>NEFSASFKGTDIQEFINIVGRNLEKT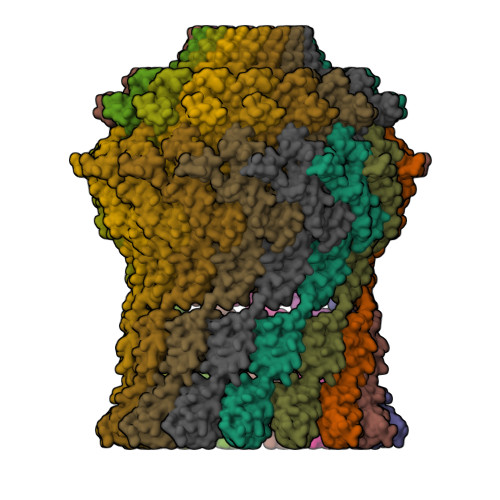IIVDPSVRGKVDVRSFDTLNEEQYYSFFLSVLEVYGFAVVEMDNGVLKVIKSKDAKTSAIPVLSGEERANGDEVITQVVAVKNVSVRELSPLLRQLIDNAGAGNVVHYDPANIILITGRAAVVNRLAEIIRRVDQAGDKEIEVVELNNASAAEMVRIVEALNKTTDAQNTPEFLKPKFVADERTNSILISGDPKVRERLKRLIKQLDVEMAAKGNNRVVYLKYAKAEDLVEVLKGVSENLQAEKGTGQPTTSKRNEVMIAAHADTNSLVLTAPQDIMNAMLEVIGQLDIRRAQVLIEALIVEMAEGDGINLGVQWGSLESGSVIQYGNTGASIGNVMIGLEEAKDTTQTKAVYDTNNNFLRNETTTTKGDYTKLASALSSIQGAAVSIAMGDWTALINAVSNDSSSNILSSPSITVMDNGEASFIVAEEVPVITGSTAGSNNDNPFQTVDRKEVGIKLKVVPQINEGNSVQLNIEQEVSNVLGANGAVDVRFAKRQLNTSVMVQDGQMLVLGGLIDERALESESKVPLLGDIPLLGQLFRSTSSQVEKKNLMVFIKPTIIRDGVTADGITQRKYNYIRAEQLFRAEKGLRLLDDASVPVLPKFGDDRRHSPEIQAFIEQMEAKQ[15x]>[3x]MTDDKKKGKFIVFEGLDRSGKSTQSKLLVEYLKNNNVEVKHLYFPNRETGIGQIISKYLKMENSMSNETIHLLFSANRWEHMNEIKSLLLKGIW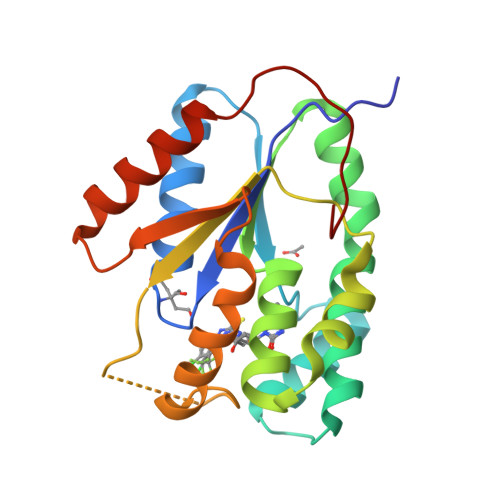VVCDRYAYSGVAYSSGALNLNKTWCMNPDQGLIKPDVVFYLNVPPNYAQNRSDYGEEIYEKVETQKKIYETYKHFAHEDYWINIDATRKIEDIHNDIVKEVTKIKVEPEEFNFLWS> DLPPVAKAAQVVNQTLQLDDSYPDLDSYCRPGASSDYEMQSSDSSWAPFHVVRHHNIPDKVFEHLNAGEVFTKLGLFAEIGYAWASIDSSLFLWDYTHPNPELIGYEEATHTITAVALVPPKPGVFVKTITHVLVVATTSEIILLGVSATPTPSGSKSLTLYSTRMSVHRGGSDVSFIVGTKDGRIFLGGESDTDIHEIFYQQEERWFSSRCGKINHSHPFGSRQQEWLRGLYVDDTRNLLYSLSNRSTIRTYHMEGPEKLTKVIEKDKTSCLRDFAHMADSSPLFTDKTNIVALSPIPATEASKLHLMALTDTGCRLFLSATSSASYTMGGATSLAPQSMQLQFVKFPPRESPTRIRTLNGQIIDSQLDKTSRALDPSALGFRFSPGYFFDVVR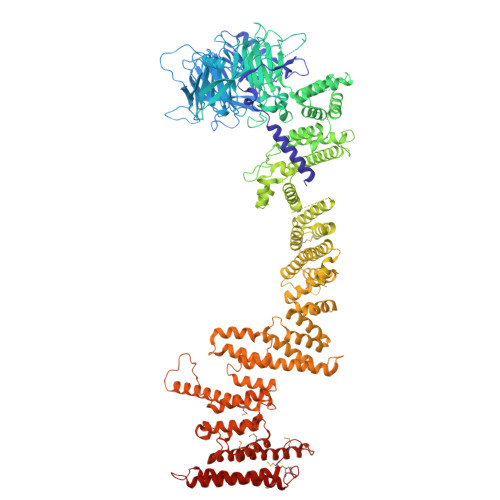KHPNQDMLFVSAPDTGRIKVTQPASALKYFEQGTWIELENGNRTIEIGLTTAPFAAAKQPLGFGNELAVQFDQVPGEFAVLTNTGVHIVRRRRLVDIFAKALGNCVSASDDALEREVRKFINQYGRVETIAAALAVACGQGSDLRTGTGRGMDRNTENLARAAFIEYGGQPRLAASDGKQSVSESVRLSSRHDALALYLTRLVRTLWKAKVVQVGSGSDISSTIPTLVTIQENVERLRNFLEANKSTIQGLAPPSERLFGRQEDIANQKEHQALHALQKLMESISEGISFVLMLFDERVSDIYARLDAVSQQQLKDLTYEQLFSQTPGKELAKVLVKAIVNRNIASGANVETVADALRRRCGSFCAPDDVVTFKAQEQLQRASEQAHNAPVLRALLAESLRLFEQVAGSLTPANLTTAVEQMISLKYYAGAIQLCLTVAQQKDRGNTALSWVNDGKPANDSRKKAFDERKICYNLIHQVLDKLESDFAGEPELVDGRPTLAATKRMEAYNVVNDSSDEVFHFDMYEWYIEKGWTDRILSIDSPHVITYLQRLAETDFRHAELLCRFYTTRSRFFEAAQVQTNLAKSDLNISLKDRIILLSRAKGNASVNTIGISRQQQQQLNHEASELLEIAHIQDDLLERLVADPRIPEERKAEIEEFLDGPIRTLTDLFNDYADQANYYDLCLLIFHAADFHNPRTIMDTWNNLINQSHFEAEQRREYWEIVQAGGDLPAGVIAPIAEPPLPYVYVSQQIQLIAHRTSLDSLIFPVNSLLPVVCAYAINNGQDASIGADPCWPIQLFLNLGVPHALMVQVLENVLDTQEAPFTGRRRKLVVQWIAMAVDMWVREVERRGAMAAAAASGASGSEAVMGSWVSELLGRADQVLTQIAGTGATLRGGAASDAEEIASLRRTVKGLKRSVDMLLGGEMARMSFFR>CCGGCGCCGG[4x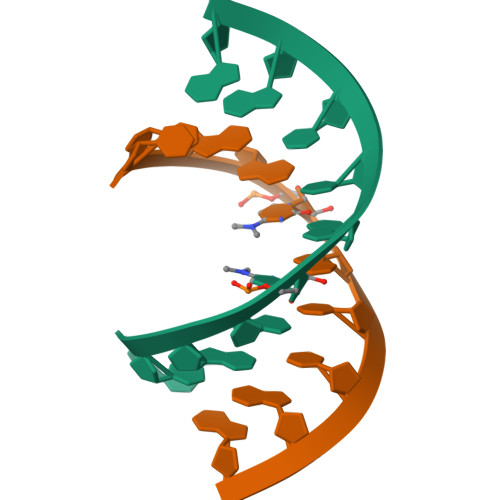]RIBOSTAMYCIN | C17 H34 N4 O10 | 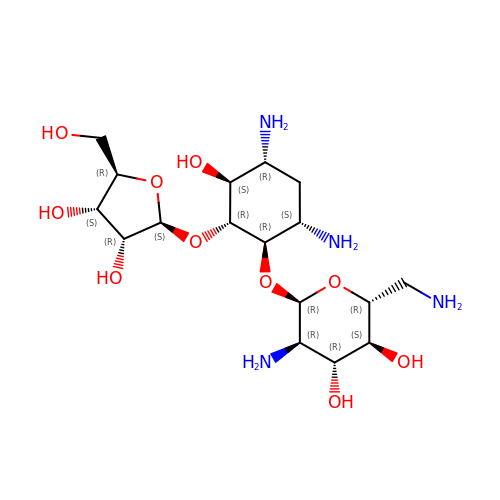NSKGQURZWSPSBC-VVPCINPTSA-N> VEWTDKERSIISDIFSHMDYDDIGPKALSRCLVVYPWTQRYFSGFGNLYNAEGIMSNANVAAHGIKVLHGLDRGMKNMDNIADAYTDLSTLHSEKLHVDPDNFKLLSDCITIVLAAKMGHAFTAETQGAFQKF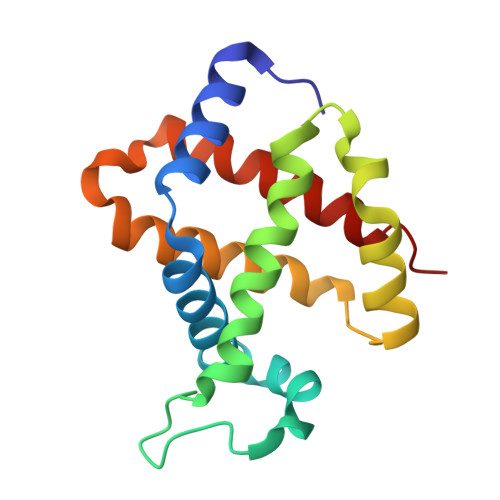LAAVVSALGKQYH> SSSVVLDSENGVETESRKLPSSKYKGVVPQPN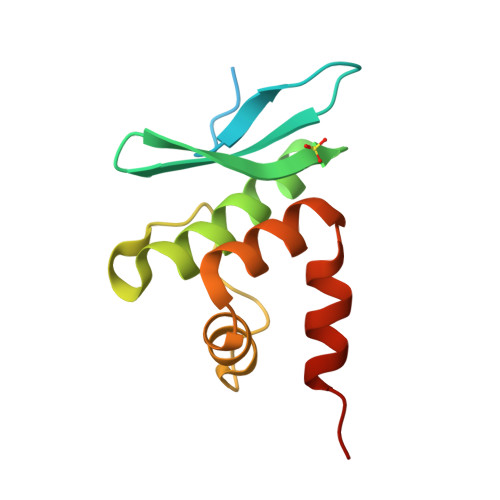GRWGAQIYEKHQRVWLGTFNEEEEAASSYDIAVRRFRGRDAVTNFKSQVDGNDAESAFLDAHSKAEIVDMLRKHTYADEFEQSRRKFVNG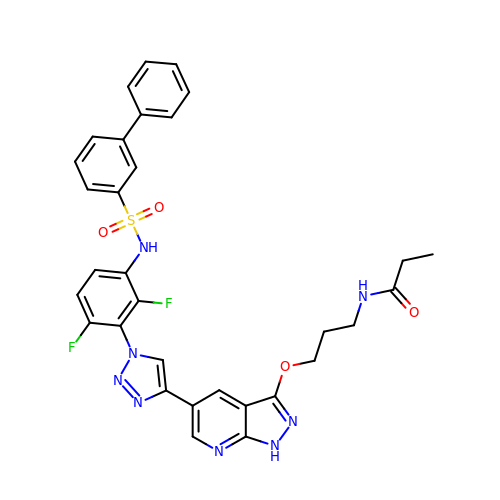~{N}-[3-[[5-[1-[2,6-bis(fluoranyl)-3-[(3-phenylphenyl)sulfonylamino]phenyl]-1,2,3-triazol-4-yl]-1~{H}-pyrazolo[3,4-b]pyridin-3-yl]oxy]propyl]propanamide | C32 H28 F2 N8 O4 S | CWIXDXZUNUCBPW-UHFFFAOYSA-N> MHHHHHHGKNHAGSPGCEESAAGKEKLPKMRLPTRSDMICGYACLKGTAAMRNTKRGSWYIEALAQVFSERACDMHVADMLVKVNALIKDREG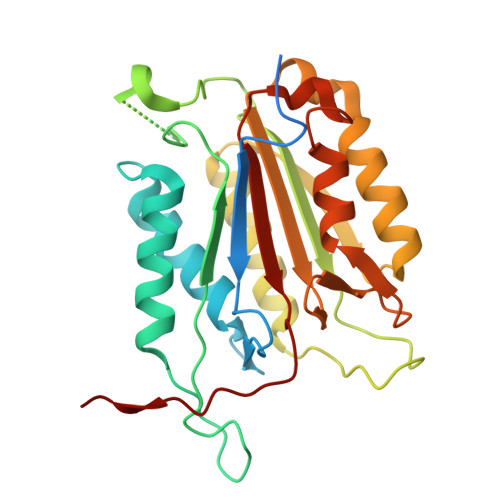YAPGTEFHRCKEMSEYCSTLCRHLYLFPGGGVKPCTPEFYQTHFQLAYRLQSRPRGLALVLSNVHFTGEKELEFRSGGDVDHSTLVTLFKLLGYDVHVLCDQTAQEMQEKLQNFAQLPAHRVTDSCIVALLSHGVEGAIYGVDGKLLQLQEVFQLFDNANCPSLQNKPKMFFIQACRGDETDRGVDQQD> MGAAVTLNRIKIAPGIADIRDKYMELGFNYPEYNRAVKFAEESYTYYYETSPGEIKPKFCLIDGMSIDHCSSFIVPEFAKQYVLIHGEPCSSFKFRPGSLIYYQNEVTPEYIKDLKHATDYIASGQRCHFIKKDYLLGDSDSVAKCCSKTNTKHCPKIFNNNYKTEHCDDFMTGFCRNDPGNPNCLEWLRAKRKPAMSTYSDICSKHMDARYCSEFIRIIRPDYFTFGDTALYVFCNDHKGNRNCWCANYPKSNSGDKYLGPRVCWLHECTDESRDRKWLYYNQDVQRTRCKYVGCTINVNSLALKNSQAELTSNCTRTTSAVGDVHPGEPVVKDKIKLPTWHHHHHH;> MGGGVSVELPKRDPPPGVPTDEMLLNVDKMHDVIAPAKLLEYVHIGPLAKDKEDKVKKRYPEFRLVNTGPGGLSALLRQSYNGTAPNCCRTFNRTHYWKKDGKISDKYEEGAVLESCWPDVHDTGKCDVDLFDWCQGDTFDRNICHQWIGSAFNRSNRTVEGQQSLINLYNKMQTLCSKDASVPICESFLHHLRAHNTEDSKEMIDYILRQQSADFKQKYMRCSYPTRDKLEESLKYAEPRECWDPECSNANVNFLLTRNYNNLGLCNIVRCNTSVNNLQMDKTSSLRLSCGLSNSDRFSTVPVNRAKVVQHNIKHSFDWSHP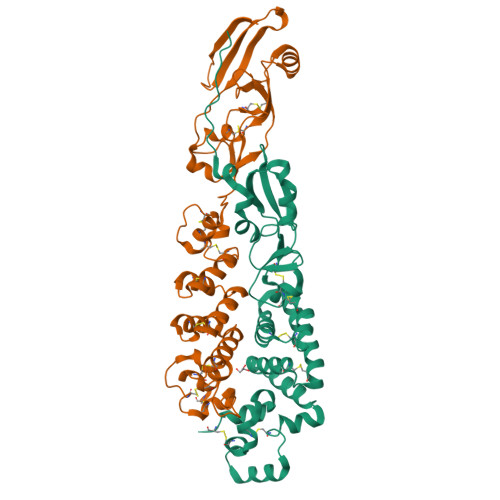QFEK> NKREETDMRDFFVITNSEYTFAGVHYAKGAVLHVSPTQKRAFWVIADQENFIKQVNKN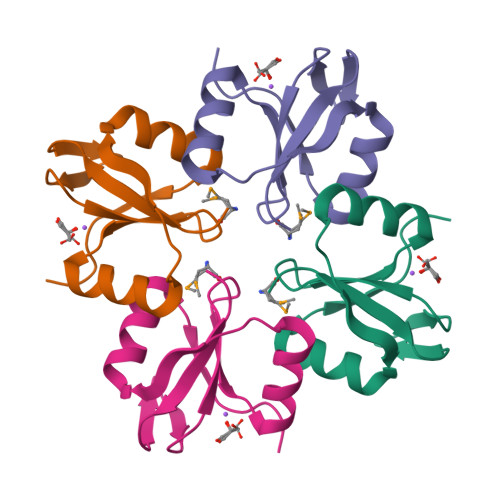IEYVEKNASPAFLQRIVEIYQVKFEGKNVH>ADKELKFLVVDDESTMRRIVRNLLKELGFNNVEEAEDGVDALNKLQAGGYGFVISDWNMPNMDGLELLKTIRAD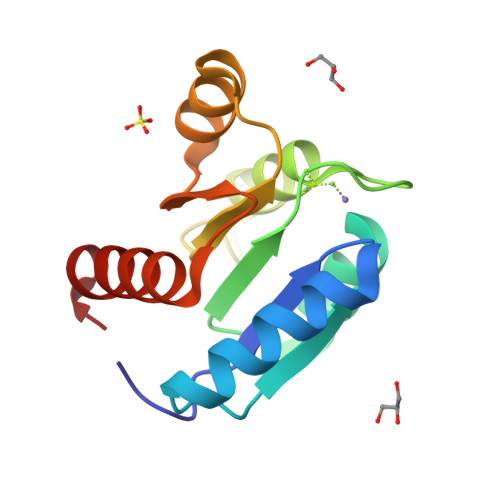GAMSALPVLMVTARAKKENIIAAAQAGASGYVVKPFTAATLEEKLNKIFEKLGM[2x]>MEVRNMVDYELLKKVVEAPGVSGYEFLGIRDVVIEEIKDYVDEVKVDKLGNVIAHKKGEGPKVMIAAHMDQIGLMVTHIEKNGFLRVAPIGGVDPKTLIAQRFKVWIDKGKFIYGVGASVPPHIQKPEDRKKAPDWDQIFIDIGAESKEEAEDMGVKIGTVITWDGRLERLGKHRFVSIAFDDRIAVYTILEVAKQLKDAKADVYFVATVQEEVGLRGARTSAFGIEPDYGFAIDVTIAADIPGTPEHKQVTHLGKGTAIKIMDRSVICHPTIVRWLEELAKKHEIPYQLEILLGGGTD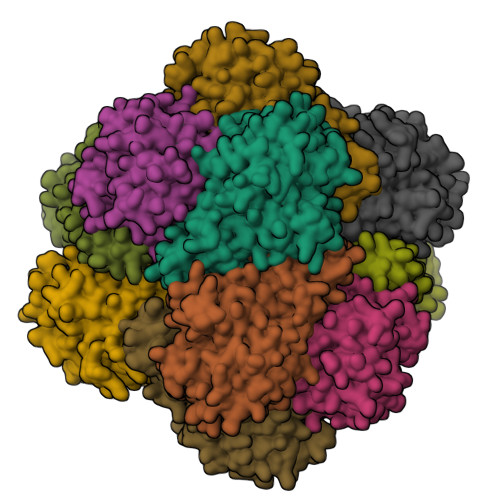AGAIHLTKAGVPTGALSVPARYIHSNTEVVDERDVDATVELMTKALENIHELKI[12x]>[6x]FGSICAFTASRTFPNGFTVTEEFADADPIDSPPFAAADTGAGLNGDMVVWNRANILEVVVNVIPNTEGERNLAVLLDANRTGKDKSGARDVVGLVVAMPDGSKITCTNGTPIDGVLINAVASVGRLKTKPYRFRFEKVIKAGTS;> MISQSRYIRIISGVGAAAPVAGRKLILRVMTTNNVIPPGIVIEFDNANAVLSYFGAQSEEYQRAAAYFKFISKSVNSPSSISFARWVNTAIAPMVVGDNLPKTIADFAGFSAGVLTIMVGAAEQNITAIDTSAATSMDNVASIIQTEIRKNADPQLAQATVTWNQNTNQFTLVGATIGTGVLAVAKSADPQDMSTALGWSTSNVVNVAGQSADLPDAAVAKSTNVSNNFGSFLFAGAPLDNDQIKAVSAWNAAQNNQFIYTVATSLANLGTLFTLVNGNAGTALNVLSATAANDFVEQCPSEILAATNYDEPGASQNYMYYQFPGRNITVSDDTVANTVDKSRGNY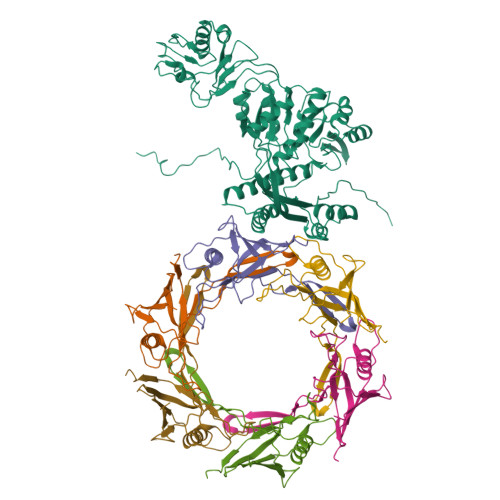IGVTQANGQQLAFYQRGILCGGPTDAVDMNVYANEIWLKSAIAQALLDLFLNVNAVPASSTGEAMTLAVLQPVLDKATANGTFTYGKEISAVQQQYITQVTGDRRAWRQVQTLGYWINITFSSYTNSNTGLTEWKANYTLIYSKGDAIRFVEGSDVMI> MRLEQLQAFLAIAETGSFQKAASKCGVTQST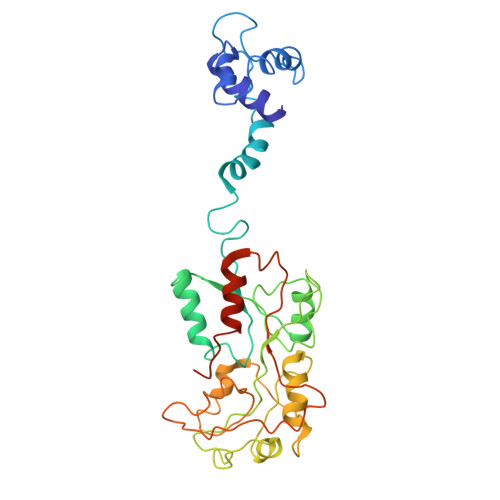ISRQIQSLEADLGLELFHRTNHSKLTLGGERLLPRARKICLEWETATQELGDLIAGKQPELCIAAIHSLCGSYLPPVLQKFCRDYPEVQLRVTSLGSDRALKVLKDGLVDLAIVMNNRFLTTGRDMVVEVLYDEPIELLTAANHPLAAYERVPWSELVRYPQVVFKDGYGMQRLVQEKFERLEATLQAALEVNTLDAFRGVVRQGELIALLPSSALVEARLDPTLAVRPLANSALPENSGLTRRVVMVTTQDRLQIPPIKHFWQLVRENIPPIVERQRSAS> QESTHIYTKEEVSSHTSPETGIWVTLGSEVFDVTEFVD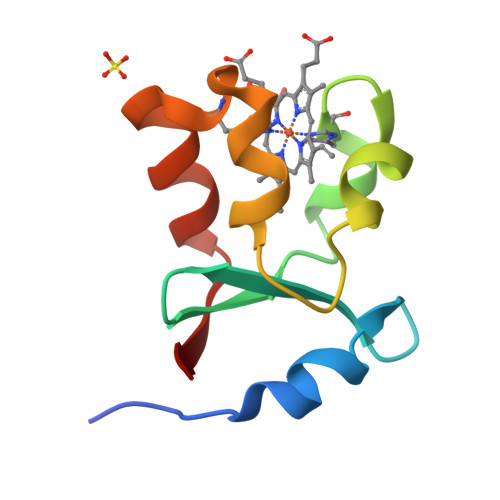LHPGGPSKLMLAAGGPLEPFWALYAVHNQSHVRELLAQYKIGEL> GELG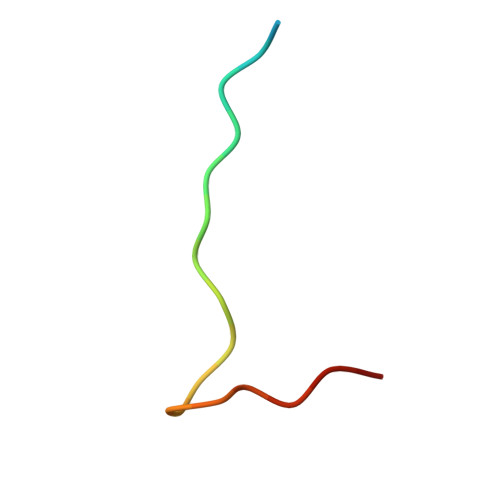RLVYLLDGPGYDPIHCD Orthologous proteins to ependymin called ependymin-related proteins (EPDRs) have been found to exist in various tissues from sea urchins to humans, yet their functional role remains to be revealed. All of the EPDR1s fold into a dimer using a monomeric subunit that is mostly made up of two stacking antiparallel β-sheets with a curvature on one side, resulting in the formation of a deep hydrophobic pocket. All six of the cysteine residues in the monomeric subunit participate in the formation of three intramolecular disulfide bonds. The EPDR1 fold is very similar to the folds of bacterial VioE and LolA/LolB, which also use a similar hydrophobic pocket for their respective functions as a hydrophobic substrate-binding enzyme and a lipoprotein carrier, respectively.

Buried surface areas (BSAs) of ∼1900 and ∼200 Å2 (both per subunit from PISA analysis; Krissinel & Henrick, 2007) were created between the subunits. Judging from the sizes of these areas, the smaller interface burying ∼200 Å2 is only a lattice contact, while the dimeric surface burying ∼1900 Å2 is likely to be a crucial interaction mode with physiological relevance. In this mode of inter­action, the second of the two β-sheet layers (β2–β1–β11–β10–β9–β8–β7) mediates the dimeric interface. The structure of human EPDR1 was subjected to a fold-similarity search using the DALI server, and the top two highest scoring structures were found to be the bacterial VioE (r.m.s.d. = 3.7 Å; Z-score = 14.6) and the bacterial LolA (r.m.s.d. = 4.0 Å; Z-score = 12.3). Also, in a recent structure of human EPDR1 that preceded our study, a ligand was observed in this cavity and was also modeled as an extended PEG chain from the crystallization condition. It is interesting to note that we do not see any electron density for any ligand in the same region despite the fact that PEGs were used to crystallize the human and frog EPDR1s. Because the displacement of 1,8-ANS by fatty acids is often used to assess the binding of fatty acids to fatty-acid-binding proteins, a similar approach was made using human EPDR1 and the fatty acids caproic acid (C6), lauric acid (C12) and stearic acid (C18). The displacement assays suggested that smaller fatty acids more preferably interact with human EPDR1.

>[4x]ADPHHHHHHHHAPRPCQAPQQWEGRQVMYQQSSGRNSRALLSYDGLNQRVRVLDERKALIPCKRLFEYILLYKDGVMFQIDQATKQCSKMTLTQPWDPLDIPQNSTFEDQYSIGGPQEQITVQEWSDRKSARSYETWIGIYTVKDCYPVQETFTINYSVILSTRFFDIQLGIKDPSVFTPPSTCQMAQLEKMSEDCSW>GTSTQTKAGSLTIVGTGIESIGQMTLQALSYIEAAAKVFYCVIDPATEAFILTKNKNCVDLYQYYDNGKSRLNTYTQMSELMVREVRKGLDVVGVFYGHPGVFVNPSHRALAIAKSEGYRARMLPGVSAEDCLFADLCIDPSNPGCLTYEASDFLIRDRPVSIHSHLVLFQVGCVGIADFNFTGFDNNKFGVLVDRLEQEYGAEHPVVHYIAAMMPHQDPVTDKYTVAQLREPEIAKRVGGVSTFYIPPKARKASNLDIIRRLELLPAGQVPDKKARIYPANQWEPDVPEVEPYRPSDQAAIAQLADHAPPEQYQPLATSKAMSDVMTKLALDPKALADYKADHRAFAQSVPDLTPQERAALELGDSWAIRCAMKNMPSSLLDAARESGEEASQNGFPWVIVVGVIGVIG[2x]

While chemical methylation of an amide bond uses a strong base to generate the imidate, OphA, the precursor protein of the fungal peptide macrocycle omphalotin A, self-hypermethylates amides at pH 7 using S-adenosyl methionine (SAM) as cofactor. Omphalotin A derives from the C terminus of the OphA protein, and it is the OphA protein that methylates its own C terminus using S-adenosyl methionine (SAM). The structure of OphA reveals a complex catenane-like arrangement in which the peptide substrate is clamped with its amide nitrogen aligned for nucleophilic attack on the methyl group of SAM. Here, we report the structure of the peptide amide methyltransferase OphA including complexes with cofactor [SAM and S-adenosyl homocysteine (SAH)], cofactor analog, substrate, and product.

A second variant of OphA, truncated at Gly411 (OphAΔC6), containing the core peptide, is catalytically active with methylation of up to seven residues. Complete methylation of OphAΔC6 occurs over a similar time frame as native OphA, suggesting that this truncated version is a valid model for the full-length enzyme. The structure is otherwise essentially identical to OphAΔC18 (rmsd of 0.6 Å over 688 Cα atoms) with no notable conformational changes of the residues that comprise the binding site. For ease of discussion, we split the protein into three sections: the N-terminal (methyltransferase) domain, the clasp domain, and the C-terminal substrate peptide. Inspection of the experimental maps reveals that while the positions of substrate backbone atoms are unambiguous, density for the side chains is suggestive of some heterogeneity in the register of the bound substrate peptide. The location of the cofactor relative to the protein is identical in both the OphAΔC18 and OphAΔC6 complexes. The peptide carbonyl at i−3 hydrogen-bonds to the side chain of Tyr63, at i−2 to the side chain of Tyr98, and at i−1 to both Tyr66 and Tyr76. The side chains at i−1 and i−3 both sit in large hydrophobic pockets, while the side chains at i−4, i−5, and i−6 are exposed to solvent. In both solution and crystal, neither Ile410 nor Gly411 of OphAΔC6 is methylated. The substrate side chains do not make any specific contacts with OphA, consistent with the protein’s ability to methylate different residues (Gly, Val, Ile, Met, Thr, and Ala).> IFPKQYPIINFTTAGATVQSYTNFIRAVRGRLTTGADVRHEIPVLPNRVGLPINQRFILVELSNHAELSVTLALDVTNA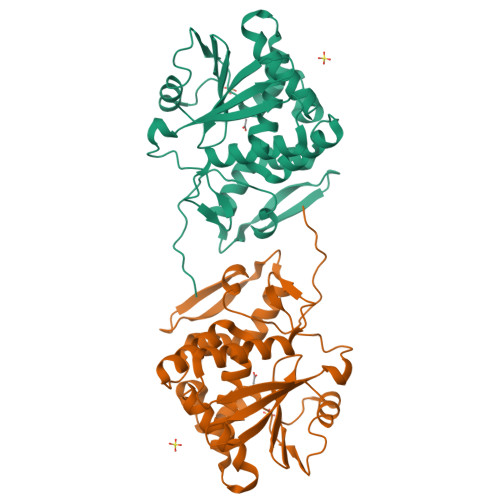YVVGYRAGNSAYFFHPDNQEDAEAITHLFTDVQNRYTFAFGGNYDRLEQLAGNLRENIELGNGPLEEAISALYYYSTGGTQLPTLARSFIICIQMISDAARFQYIEGEMRTRIRYNRRSAPDPSVITLENSWGRLSTAIQESNQGAFASPIQLQRRNGSKFSVYDVSILIPIIALMVYRCAPPPSSQF>LTLGNTTSSVILTNYMDTQYYGEIGIGTPPQTFKVVFDTGSSNVWVPSSKCSRLYTACVYHKLFDASDSSSYKHNGTELTLRYSTGTVSGFLSQDIITVGGITVTQMFGEVTEMPALPFMLAEFDGVVGMGFIEQAIGRVTPIFDNIISQGVLKEDVFSFYYNRDSLGGQIVLGGSDPQHYEGNFHYINLIKTGVWQIQMKGVSVGSSTLLCEDGCLALVDTGASYISGSTSSIEKLMEALGAKKRLFDYVVKCNEGPTLPDISFHLGGKEYTLTSADYVFQESYSSKKLCTLAIHAMDIPPPTGPTWALGATF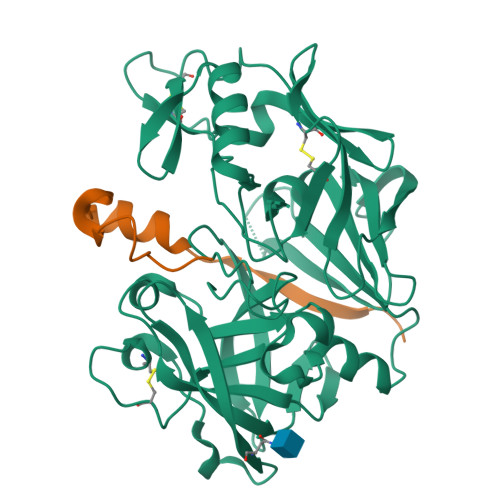IRKFYTEFDRRNNRIGFALAR[2x];>LPTDTTTFKRIFLKRMPSIRESLKERGVDMARLGPEWSQPMKR[2x]(2E,6E)-3,7,11-trimethyldodeca-2,6,10-trien-1-ol | C15 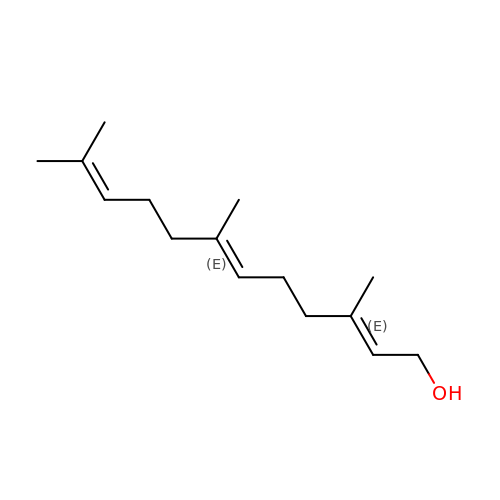H26 O | CRDAMVZIKSXKFV-YFVJMOTDSA-N>[2x]GHSVEIIVRDNCGSCVRVKAQILPIVEAAGIKLTERNVDQDAS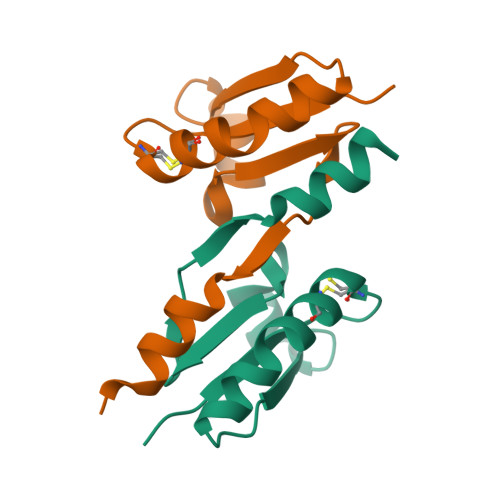LKLEFGDRVPVILVDDEEFACWEVDNDELANALLLEHHHHHH> EAGEFFIRAGTATVRPTEGSDNVLGSLGSFNVSNNTQLGLTFTYMATDNIGVELLAATPFRHKVGTGPTGTIATVHQLPPTLMAQWYFGDAQSKVRPYVGAGINYTTFFNEDFNDTGKAAGLSDLSLKDSWGAAGQVGLDYLINRDWLLNM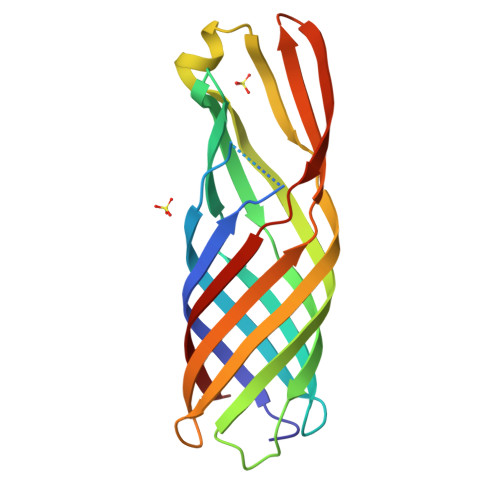SVWYMDIDTDVKFKAGGVDQKVSTRLDPWVFMFSAGYRF>[2x]MR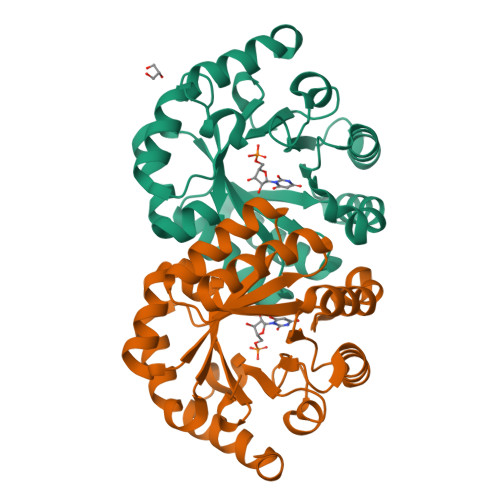SRRVDVMDVMNRLILAMDLMNRDDALRVTGEVREYIDTVKIGYPLVLSEGMDIIAEFRKRFGCRIIADFKVADIPETNEKICRATFKAGADAIIVHGFPGADSVRACLNVAEEMGREVFLLTEMSHPGAEMFIQGAADEIARMGVDLGVKNYDGPSTRPERLSRLREIIGQDSFLISPGVGAQGGDPGETLRFADAIIVGRSIYLADNPAAAAAGIIESIKDLLNP>MALSANSDAVTYAKAANTRTAAETGDRIEWVKLSLAFLPLATPVSDAKVLTGRQKPLTEVAIIIAEIRSRDGFEGVGFSYSKRAGGQGIYAHAKEIADNLLGEDPNDIDKIYTKLLWAGASVGRSGMAVQAISPIDIALWDMKAKRAGLPLAKLLGAHRDSVQCYNTSGGFLHTPLDQVLKNVVISRENGIGGIKLKVGQPNCAEDIRRLTAVREALGDEFPLMVDANQQWDRETAIRMGRKMEQFNLIWIEEPLDAYDIEGHAQLAAALDTPIATGEMLTSFREHEQLILGNASDFVQPDAPRVGGISPFLKIMDLAAKHGRKLAPHFA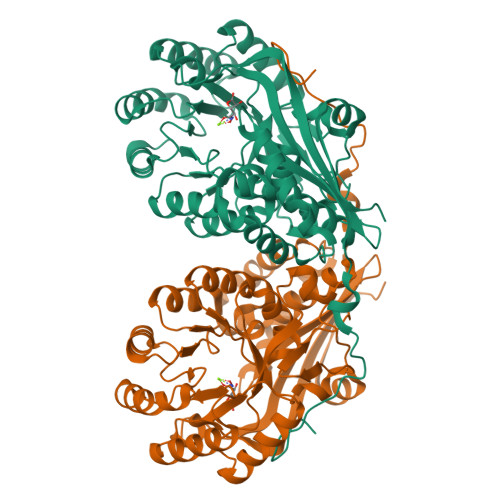MEVHLHLSAAYPLEPWLEHFEWLNPLFNEQLELRDGRMWISDRHGLGFTLSEQARRWTQLTCEFGKRP[6x]>[8x]VSFDSLSPQELAALHARHQQDYAALQGMKLALDLTRGKPSAEQLDLSNQLLSLPGDDYRDPEGTDTRNYGGQHGLPGLRAIFAELLGIAVPNLIAGNNSSLELMHDIVAFSMLYGGVDSPRPWIQEQDGIKFLCPVPGYDRHFAITETMGIEMIPIPMLQD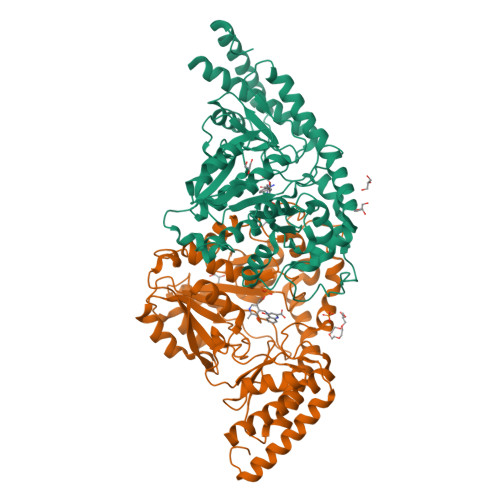GPDVDLIEELVAVDPAIKGMWTVPVFGNPSGVTYSWETVRRLVQMRTAAPDFRLFWDNAYAVHTLTLDFPRQVDVLGLAAKAGNPNRPYVFASTSKITFAGGGVSFFGGSLGNIAWYLQYAGKKSIGPDKVNQLRHLRFFGDADGVRLHMLRHQQILAPKFALVAEVLDQRLSESKIASWTEPKGGYFISLDVLPGTARRTVALAKDVGIAVTEAGASFPYRKDPDDKNIRIAPSFPSVPDLRNAVDGLATCALLAATETLLNQGLASSAPNVR2-[(2-amino-9-methyl-6-oxo-6,9-dihydro-1H-purin-8-yl)sulfanyl]-N-phenylacetamide 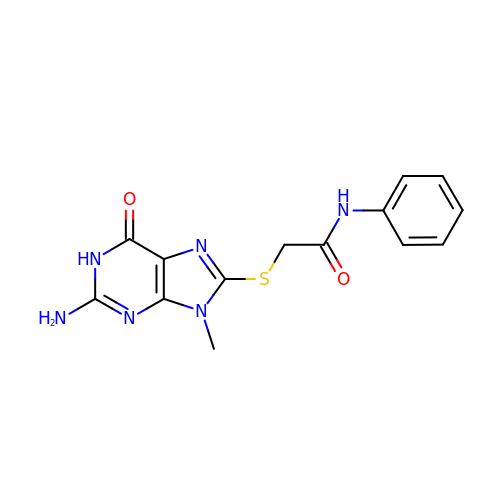| C14 H14 N6 O2 S | ZDOIVRCQPDEDGR-UHFFFAOYSA-N> MTTLLNPYFGEFGGMYVPQILMPALNQLEEAFVSAQKDPEFQAQFADLLKNYAGRPTALTKCQNITAGTRTTLYLKREDLLHGGAHKTNQVLGQALLAKRMGKSEIIAETGAGNHGVAS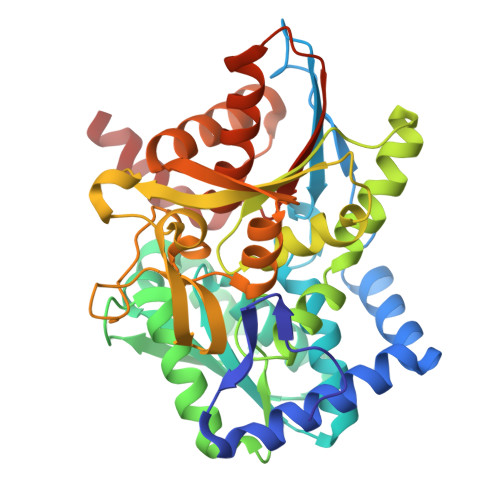ALASALLGLKCRIYMGAKDVERQSPNVFRMRLMGAEVIPVHSGSATLKDACNEALRDWSGSYETAHYMLGTAAGPHPYPTIVREFQRMIGEETKAQILDKEGRLPDAVIACVGGGSNAIGMFADFINDTSVGLIGVEPGGHGIETGEHGAPLKHGRVGIYFGMKAPMMQTADGQIEESYSISAGLDFPSVGPQHAYLNSIGRADYVSITDDEALEAFKTLCRHEGIIPALESSHALAHALKMMREQPEKEQLLVVNLSGRGDKDIFTVHDILKARGEI>[2x]GGCUCUGGAGAGAACCG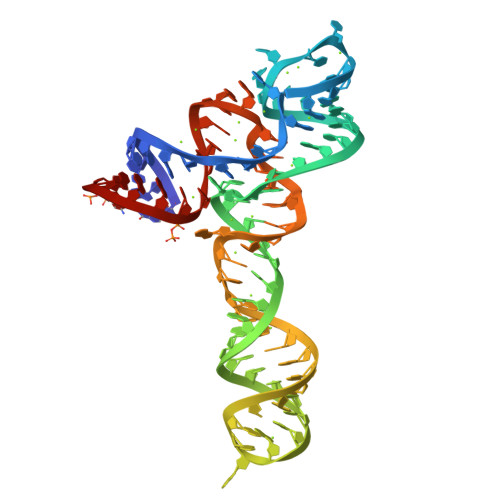UUUAAUCGGUCGCCGAACGAGCAAGCUCUGCGGAAACGCAGAGUGAAACUCUGAGGCAAAAGGACAGAGUC> MITVPHSRKVELDEIDRAILRLLQEDGRMSYSEISRRINVPESTVRARVNRLVKEGVIRKF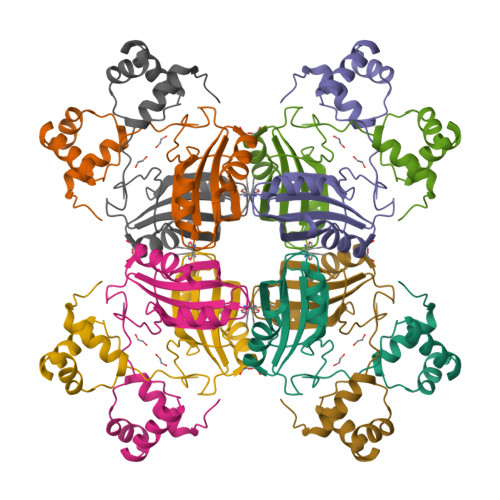AALINPFKAGYEIVAFIAVDAEPAKVKQVVEELAKFPEVDVLGIVTGAHDIFMQVTVKDLQELERFILEKMAKIDGIKSTETSILTSVKKWGYARVFHHHHHH> MSNQQGPEDNNLEDDMAYLPADHPLLAKLQIDLTKQLTDEHERVDQKLIEIDANLKKLEKTKEDIGVRLYSVQQQLAENQMNFEQAHENYNWVQKLRIEAEQKLKTESEVYDAKKKELEELRKKYLKAQDELSKLTRTLYQINEFNQQMKGQIINTKTNTYRAEENVVNLEAQKKKQDLLIDTMNEEIKRQTEQKTILTAQLISQKEETEQAKQILKEAHLEMQKIIASKKNLLERWQKSLMTMQRMDNALQAIKEALKGQQELNLQIGTELNGVNAEIRKETEIQESLEGKNKKFDYEKDYLQKKYNELQEEKSKLEAQINLLTQSLRQTETEAGRAEIDKRNIEDQMNLIETNIMKLHTETKKLWEDLVHQKSEHTTIEKTATNLNKQANQISIEIEDKSVELENLLNEIARVKIDQLNTLSQIEVLENKRREVIKEREEKEITVATYEVQIRQGHDLNEKKQHEVGRLNREHDKLSSVQSDMSRGPLEAKRNNLIRKTQELGKENDLMQREWIKKQTLLVTQNNRLNKIEEDVSQLKTKQTILEQKKLRLNNNYRIYEKDIREIQNALKNLRNEMNKLNDAIYRNKEKQQKLDNENFNIKSEFVEKLKELEKESVKLEVEIDRLKEEKADLLAEIVESERQILLWERKIQLEKEMQDALDPTVGQTEIQELKREIHRMELRLDDLRKKQEAIIAEMERAVYKRETIQLKYMNKDKTFSNSNSMSQKSSSISAASDNSAQITKKIAQLKTTLNQTTRNAEQMEKAIKNKKIELDDLNAQIEGNNDNLQKLESDCYNKNIELTKHKLERSTNILSISCMQNKAKKLEDLV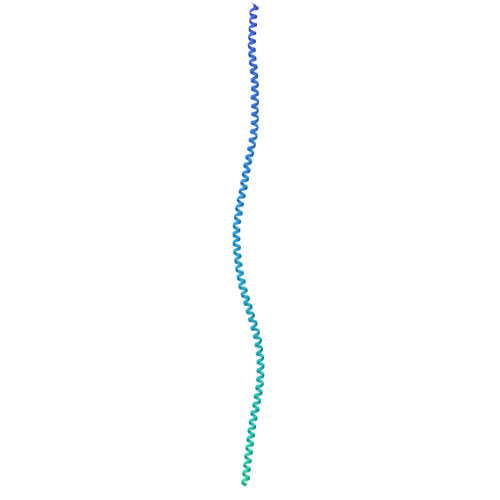AGKARLSVPEATLMTKYEELRDKNQEIKEALQKLCDDAPQYVEVLNYLIDLNVGDDDEDQEQ>[2x]MPKAKAKTKNTEIISPHHYVYPNTTTLKNKYGIKNLNAFLEKCSHDTAKAMINLREESLPEYFDTAYLCHIHQQLFKNTFEWAGYLRHIPFTFADGTTAAMPEMKRTGWKNAFAIGDEIQEGLQRLDQTLAEKNNLQGLTREEFNSEAIELFNSLNQLHPFREGNGRTQRLFFENLAKAAGHQLNFSLITKERMMVASVAVAEN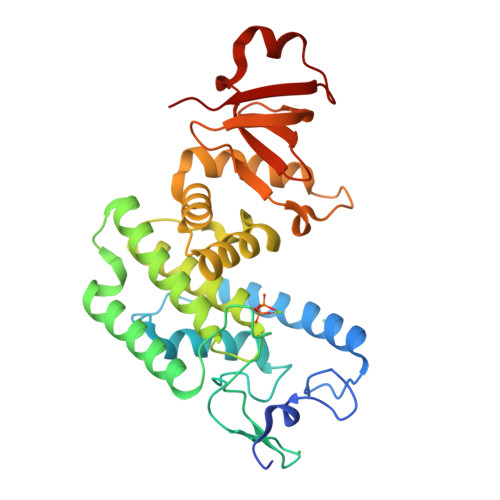GDLEPMQHLFEDISNPEKIRLLKEFMHTMKNTGRNVNDRPVMVAKEGETYTGTYRGAGLEGFALNVKGAYIIGNIDHLPPEQLKILKPGDKITFTAPK>MAFELPKLPYAFDALEPHFDKETMEIHHDRHHNTYVTKLNAAVEGTDLESKSIEEIVANLDSVPANIQTAVRNNGGGHLNHSLFWELLSPNSEEKGTVVEKIKEQWGSLEEFKKEFADKAAARFGSGWAWLVVNNGQLEIVTTPNQDNPLTEGKTPILGLDVWEH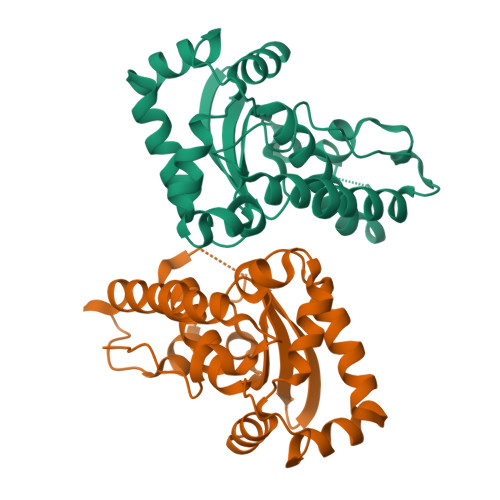AYYLKYQNKRPDYIGAFWNVVNWEKVDELYNATK[4x]{3-chloro-4-[(2-fluorophenyl)methoxy]phenyl}borinic 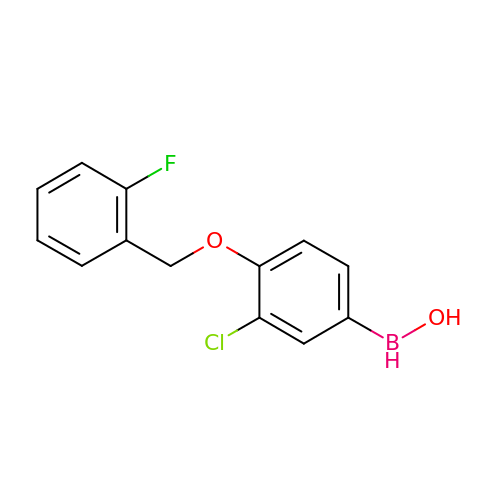acid | C13 H11 B Cl F O2 | XKCHKRXBHQBTGI-UHFFFAOYSA-N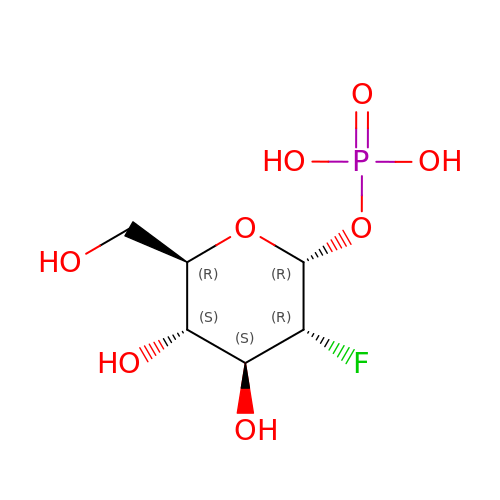2-deoxy-2-fluoro-1-O-phosphono-alpha-D-glucopyranose | C6 H12 F O8 P | LXEHNDWFCMGWAY-QZABAPFNSA-N Myo7 is a crucial component of the tripartite complex that maintains the necessary mechanical tension across the cadherin links. The Myo7 tail domain consists of two MyTH4-FERM (MF; myosin tail homology 4; band 4.1, ezrin, radixin, moesin) domains separated by an SH3 domain. Harmonin plays a pivotal role due to its ability to interact with cadherin as well as all other components of the complex. The results presented here reveal nearly identical interactions between members of the Myo7/harmonin-a/SANS:ANKS4B tripartite complexes that link cadherins to the actin-rich core in stereocilia and microvilli. Both Myo7a and Myo7b MF2 domains bind to harmonin-a PDZ3c with similar affinities via a novel mode.

Consistent with this sequence conservation, PDZ3c binds to Myo7a MF2 with ∼1 μM affinity, the same affinity as the Myo7b MF2/PDZ3c interaction. The structure of Myo7a MF2 bound to harmonin PDZ3c was determined at 2.6 Å resolution. Comparison with the PDZ3c/Myo7b MF2 structure results in an r.m.s.d. of 1.20 Å (for 411 Cα atoms) despite the low-sequence identity (51%) between the two MF2 domains and major differences in the crystal packing environments. The harmonin PDZ3c binds in the same overall manner by inserting the Cter motif into Myo7a MF2’s central FERM cavity. However, the Cter motif adopts a slightly different conformation in the two complexes, namely residues Leu549 and Thr550 interact distinctively in the two FERM cavities due to the Tyr2026Myo7a/Phe1923Myo7b variation. Such slight adaptability of the FERM groove results mainly from conformational variability in the F1 lobe. The affinities of PDZ3c for either Myo7a or Myo7b MF2 are similar despite these changes, showing that some adaptation of the binding mode in this FERM cavity can occur without much cost in affinity. However, several deafness mutations suggest the importance of this domain for the integrity of stereocilia. In light of the new structures, 25 missense mutations of Myo7a MF2 that cause deafness were mapped onto the structure to assess their potential impact on binding to partners (Supplementary Table 2 and references therein). However, mutations affecting three surface residues (K2118N, G2163S, G1982E/R) suggest a role for the surface next to the F1H2-S5 loop and the F3 lobe in making specific interactions with partners. Interestingly, these four mutations significantly weaken the interaction with PDZ3c, suggesting the importance of the Myo7a MF2/harmonin PDZ3c interactions in hearing and a functional role for harmonin-a.

> MGSSHHHHHHSSGTAEPEVRAKPYTLEEFSYDYFRPPPKHTLSRVMVSKARGKDRLWSHTREPLKQALLKKLLGSEELSQEACLAFIAVLKYMGDYPSKRTRSVNELTDQIFEGPLKAEPLKDEAYVQILKQLTDNHIRYSEERGWELLWLCTGLFPPSNILLPHVQRFLQSRKHCPLAIDCLQRLQKALRNGSRKYPPHLVEVEAIQHKTTQIFHKVYFPDDTDEAFEVESSTKAKDFCQNIATRLLLKSSEGFSLFVKIADKVLSVPENDFFFDFVRHLTDWIKKARPIKDGIVPSLTYQVFFMKKLWTTTVPGKDPMADSIFHYYQELPKYLRGYHKCTREEVLQLGALIYRVKFEEDKSYFPSIPKLLRELVPQDLIRQVSPDDWKRSIVAYFNKHAGKSKEEAKLAFLKLIFKWPTFGSAFFEVKQTTEPNFPEILLIAINKYGVSLIDPKTKDILTTHPFTKISNWSSGNTYFHITIGNLVRGSKLLCETSLGYKMDDLLTSYISQMLTAMSKQRGSRSGK;> GAMGSQDFRKYEEGFDPYSMFTPEQIMGKDVRLLRIKKEGSLDLALEGGVDSPIGKVVVSAVYERGAAERHGGIVKGDEIMAINGKIVTDYTLAEADAALQKAWNQGGDWIDLVVAVCPPKEYDDELTFF>MASSAQDGNNPLFSPYKMGKFNLSHRVVLAPMTRCRALNNIPQAALGEYYEQRATAGGFLITEGTMISPTSAGFPHVPGIFTKEQVREWKKIVDVVHAKGAVIFCQLWHVGRASHEVYQPAGAAPISSTEKPISNRWRILMPDGTHGIYPKPRAIGTYEISQVVEDYRRSALNAIEAGFDGIEIHGAHGYLIDQFLKDGINDRTDEYGGSLANRCKFITQVVQAVVSAIGADRVGVRVSPAIDHLDAMDSNPLSLGLAVVERLNKIQLHSGSKLAYLHVTQPRYVAYGQTEAGRLGSEEEEARLMRTLRNAYQGTFICSGGYTRELGIEAVAQGD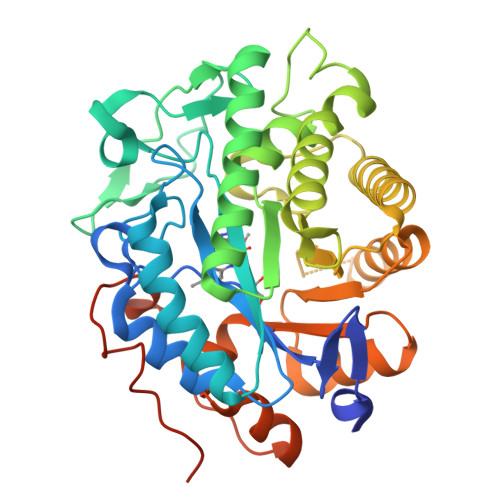ADLVSYGRLFISNPDLVMRIKLNAPLNKYNRKTFFTQDPVVGYTDYPFLQGNGSNGPLSRLLEHHHHHH[2x]>[2x]TFDERVAEVFPDMIQRSVPGYSNIISMIGMLAERFVQPGTQVYDLGCSLGAATLSVRRNIHHDNCKIIAIDNSPAMIERCRHHIDAYKAPTPVDVIEGDIRDIAIENASMVVLNFTLQFLEPSERQALLDKIYQGLNPGGALVLSEKFSFEDAKVGELLFNMHHDFKRANGYSELEISQKRSMLENVMLTDSVETHKARLHNAGFEHSELWFQCFNFGSLVALKAEDAA

Uridine at position 34 of bacterial transfer RNAs is commonly modified to uridine-5-oxyacetic acid (cmo5U) to increase the decoding capacity. The protein CmoA is involved in the formation of cmo5U and was annotated as an S-adenosyl-l-methionine-dependent (SAM-dependent) methyltransferase on the basis of its sequence homology to other SAM-containing enzymes. Mutations in the cmoB and cmoA genes result in accumulation of ho5U and mo5U, respectively, indicating that CmoB is involved in the modification of ho5U to mo5U and that CmoA is involved in the modification of mo5U to cmo5U. We have determined the structure of E. coli CmoA, a putative methyltransferase that is involved in the post-transcriptional modification of U34 in a number of bacterial tRNAs.

However, both the crystal structure of Escherichia coli CmoA at 1.73 Å resolution and mass spectrometry demonstrate that it contains a novel cofactor, S-adenosyl-S-carboxymethyl-l-homocysteine (SCM-SAH), in which the donor methyl group is substituted by a carboxy­methyl group. Unexpectedly, both molecules of CmoA contain the novel derivative S-adenosyl-S-carboxymethyl-l-homocysteine (SCM-SAH), which differs from SAM by the substitution of the methyl donor group (R = –CH3) by a carboxymethyl group (R = –CH2COOH). The negatively charged carboxylate of the carboxymethyl group interacts with the positively charged guanidinium group of Arg199 through a salt bridge with a length of 2.7 Å. However, conservation of Arg199, the key residue of CmoA that stabilizes the negative charge of the carboxyl group of the SCM-SAH cofactor, suggests that these proteins contain the SCM-SAH cofactor instead of SAM and are currently annotated incorrectly. CmoA has a Rossmann fold that comprises seven β-strands and eight α-helices. The majority of the α-helices pack against both faces of the β-sheet, although helices α2, α6 and α7 form a compact lid-like structure that sits over the region containing the SCM-SAH and renders it almost in­accessible to solvent. There are two molecules of CmoA present in the asymmetric unit that are related to each other by a noncrystallographic twofold rotational axis. In addition to an antiparallel β-­sheet formed by the β6 strands of both molecules, there are additional interactions between helix α6 of one molecule and helix α2 and strand β6 of the other molecule. Together, these interactions comprise 15 hydrogen bonds and a number of hydrophobic interactions, suggesting that the CmoA dimer present in the asymmetric unit may also represent the oligomeric state of CmoA in solution. Superpositions of CmoA with the 5-methyluridine methyltrans­ferases TrmA and RumA show that the C5 atom of the substrate uridine is neighboured by Glu164.>SDKIIHLTDDSFDTDVLKADGAILVDFWAEWCGPCKMIAPILEEIADEYQGKLTVAKLNIDQNPGTAPKYGIR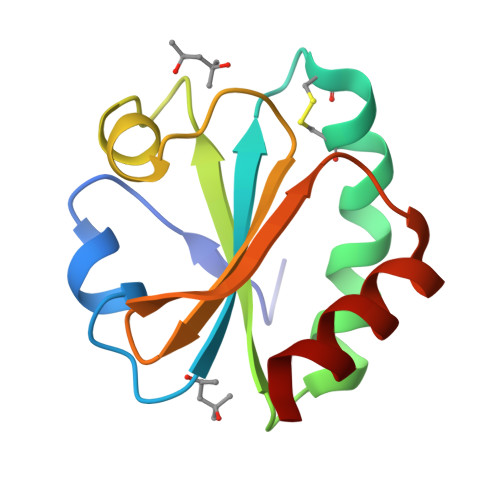GIPTLLLFKNGEVAATKVGALSKGQLKEFLDANLA[2x]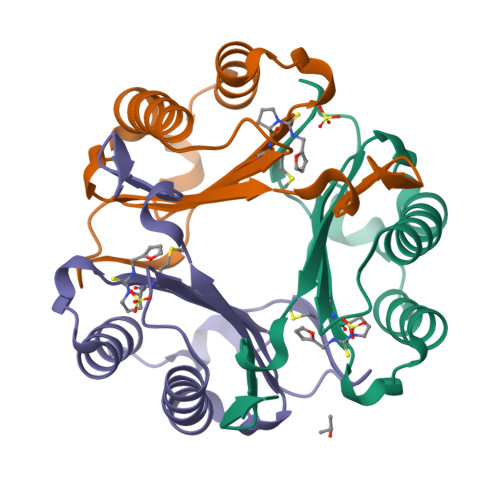>[3x]XMFIVNTNVPRASVPDGFLSELTQQLAQATGKPPQYIAVHVVPDQLMAFGGSSEPCALCSLHSIGKIGGAQNRSYSKLLCGLLAERLRISPDRVYINYYDMNAANVGWNNSTFA1,1-DIMETHYLETHYL 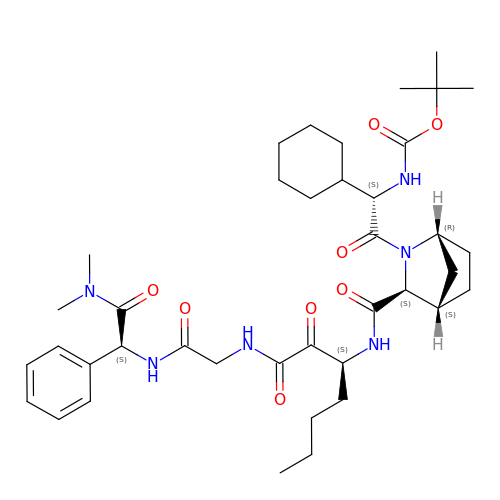[1-CYCLOHEXYL-2-[3-[[[1-[2-[[2-[[2-(DIMETHYLAMINO)-2-OXO-1-PHENYLETHYL]AMINO]-2-OXOETHYL]AMINO]-1,2-DIOXOETHYL]PENTYL]AMINO]CARBONYL]-2-AZABICYCLO[2.2.1]HEPTAN-2-YL]-2-OXOETHYL]CARBAMATE | C39 H58 N6 O8 | YGRWTFVDMXHDOB-KTARVVEZSA-N>[4x]GMNINRNKIVQLADTDTIENLTSALSQRLIADQLRLTTAESCTGGKLASALCAAEDTPKFYGAGFVTFTDQAKMKILSVSQQSLERYSAV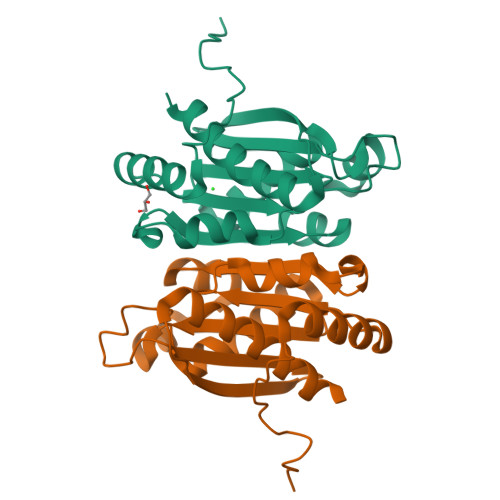SEKVAAEMATGAIERADADVSIAITGYGGPEGGEDGTPAGTVWFAWHIKGQNYTAVMHFAGDCETVLALAVRFALAQLLQLLL> MGSSHHHHHHSSGRENLYFQGHMKNVLILGAGGQIARHVINQLADKQTIKQTLFARQPAKIHKPYPTNSQIIMGDV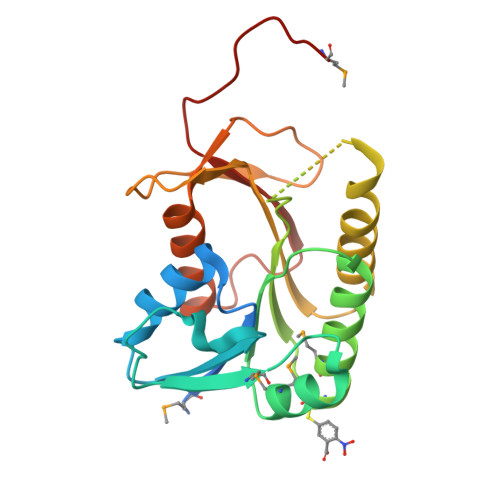LNHAALKQAMQGQDIVYANLTGEDLDIQANSVIAAMKACDVKRLIFVLSLGIYDEVPGKFVEWNNAVIGEPLKPFRRAADAIEASGLEYTILRPAWLTDEDIIDYELTSRNEPFKGTIVSRKSVAALITDIIDKPEKHIGENIGINQPGTDGDKPFFMGS>MAAIPALDPEAEPSMDVILVGSSELSSSVSPGTGRDLIAYEVKANQRNIEDICICCGSLQVHTQHPLFEGGICAPCKDKFLDALFLYDDDGYQSYCSICCSGETLLICGNPDCTRCYCFECVDSLVGPGTSGKVHAMSNWVCYLCLPSSRSGLLQRRRKWRSQLKAFYDRESENPLEMFETVPVWRRQPVRVLSLFEDIKKELTSLGFLESGSDPGQL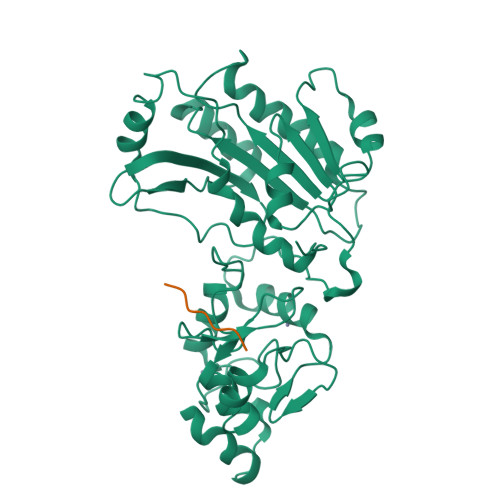KHVVDVTDTVRKDVEEWGPFDLVYGATPPLGHTCDRPPSWYLFQFHRLLQYARPKPGSPGPFFWMFVDNLVLNKEDLDVASRFLEMEPVTIPDVHGGSLQNAVRVWSNIPAIRSRHWALVSEEELSLLAQNKQSSKLAAKWPTKLVKNCFLPLREYFKYFSTELTSSL[3x];>ARTKQTA[3x]> MKCLVTGGNVKVLGKAVHSLSRIGDELYLEPLEDGLSLRTVNSSRSAYACFLFAPLFFQQYQAATPGQDLLRCKILMKSFLSVFRSLAMLEKTVEKCCISLNGRSSRLVVQLHCKFGVRKTHNLSFQDCESLQAVFDPASCPHMLRAPARVLGEAVLPFSPALAEVTLGIGRGRRVILRSYHEEEADSTAKAMVTEMCLGEEDFQQLQAQEGVAITFCLKEFRGLLSFAESANLNLSIHFDAPGRPAIFTIKDSLLDGHFVLATLSDTDS;> MHHHHHHKFRAKIVDGACLNHFTRISNMIAKLAKTCTLRISPDKLNFILCDKLANGGVSMWCELEQENFFNEFQMEGVSAENNEIYLELTSENLSRALKTAQNARALKIKLTNKHFPCLTVSVELLSMSSSSRIVTHDIPIKVIPRKLWKDLQEPVVPDPDVSIYLPVLKTMKSVVEKMKNISNHLVIEANLDGELNLKIETELVCVTTHFKDLGNPPLASESTHEDRNVEHMAEVHIDIRKLLQFLAGQQVNPTKALCNIVNNKMVHFDLLHEDVSLQYFIPALS;> MPLLTQQIQDEDDQYSLVASLDNVRNLSTILKAIHFREHATCFATKNGIKVTVENAKCVQANAAIQAGIFQEFKVQEESVTFRINLTVLLDCLSIFGSSPMPGTLTALRMCYQGYGYPLMLFLEEGGVVTVCKINTQEPEETLDFDFCSTNVINKIILQSEGLREAFSELDMTSEVLQITMSPDKPYFRLSTFGNAGSSHLDYPKDSDLMEAFHCNQTQVNRYKISLLKPSTKALVLSCKVSIRTDNRGFLSLQYAIRNEDGQICAVEYYCCPDEEVPESES;> TSKFPHLTF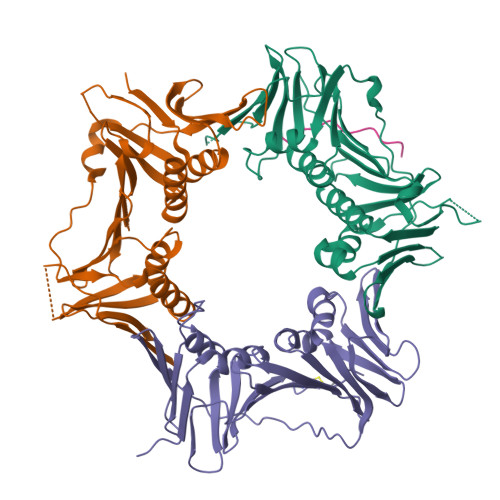ESP>MNHKVHHHHHHMLIILTGLPGVGKSTFSKNLAKILSKNNIDVIVLGSDLIRESFPVWKEKYEEFIKKSTYRLIDSALKNYWVIVDDTNYYNSMRRDLINIAKKYNKNYAIIYLKASLDVLIRRNIERGEKIPNEVIKKM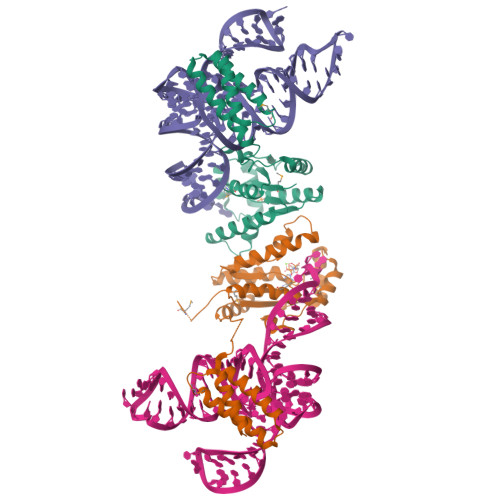YEKFDEPGKKYKWDEPFLIIDTTKDIDFNEIAKKLIEKSKEIPKFYVLEENKNKNNNISDKIDKETRKIVSEYIKSKKLDKDKIKEVVELRKEFLKKIKKMEEVDADRVLKEFKDLLNSY[2x]>SLRSDLINALYDENQKYDVCGIISAEGKIYPLGSDTKVLSTIFELFSRPIINKIAEKHGYIVEEPKQENHYPDFTLYKPSEPNKKIAIDIKTTYTNKENEKIKFTLGGYTSFIRNNTKNIVYPFDQYIAHWIIGYVYTRVATRKSSLKTYNINELNEIPKPYKGVKVFLQDKWVIAGDLAGSGNTTNIGSIHAHYKDFVEGKGIFDSEDEFLDYWRNYERTSQLRNDKYNNISEYRN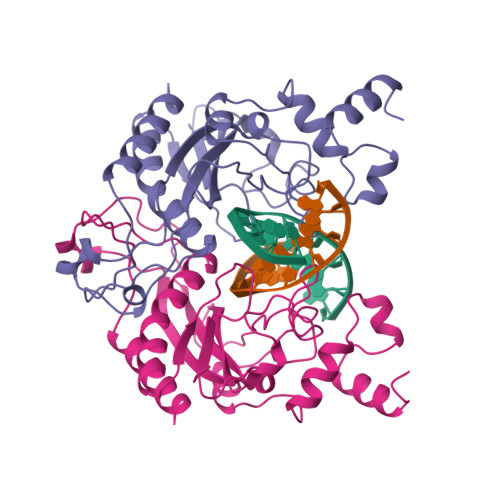WIYRGRK[2x]The bacterial flagellum can be divided into three main parts: the transmembrane basal body that acts as a rotary motor as well as the flagellar protein export machine to construct the flagellar axial structures; the long filament extending into the cell exterior to function as a helical propeller; and the hook connecting the motor and filament as a universal joint to transmit motor torque to the filament. The Salmonella hook is a short, highly curved tubular structure built by helical assembly of about 120 copies of a single protein, FlgE. The length of the hook is regulated to 55 nm ± 7 nm, and its highly curved structure and bending flexibility make it work as a universal joint, transmitting motor torque to the filament regardless of the filament orientation off-axis of the motor during run and tumble of the cell for taxis. The FlgE molecule consists of three major domains, D0, D1 and D2, that are arranged radially from the inner core to the outer surface of the tubular structure and axially from the proximal to the distal end of the hook.

We carried out the structural analysis of the flagellar hook isolated from Salmonella in the straight form by cryoEM helical image analysis and built an atomic model based on the 4.1 Å resolution map. The hook was purified from a fliK-deficient mutant strain of Salmonella, SJW880, which produces polyhooks that are structurally identical to the native hook but can grow as long as 1 µm. The final resolution of the three-dimensional image reconstruction was 4.1 Å by the criteria of a Fourier shell correlation of 0.143. In the previous model built based on a cryoEM density map, the model of domain D0 was not so accurate and that of domain Dc was missing due to limited resolution of the density map. The model of Salmonella FlgE is now complete with the full-length chain connected from the N- to the C-terminus as shown in Figure 2 in two different views. Domain D0 consists of the N- and C-terminal α-helices (Ser 1–Ala 27 and Leu 367–Arg 402, respectively) forming an antiparallel coiled coil, with the C-terminal helix facing the central channel and tilted from the hook axis by about 17°. Domain Dc is a long β-hairpin (Lys 32–Phe 60) running parallel with the N-terminal helix and with its length nearly the same as that of the N-terminal helix. Thus, domains D0 and Dc together form a compact domain, which we hereafter call domain D0-Dc. In contrast, the Dc domains (green) have close interactions in the −5-start and 11-start helical lines, making a stable tubular structure, albeit the 6-start interactions are absent. Thus, the tubular structure of the hook is stabilized and maintained mainly by the intersubunit interactions of D0-Dc domains alone in the inner core of the hook structure. Residues 38–40 in the middle of the β-hairpin of domain Dc of subunit 0 are closely interacting with the tip loop (residues 328–331) of a short β-hairpin of domain D1 of subunit −5.

> SFSQAVSGLNAAATNLDVIGNNIANSATYGFKSGTASFADMFAGSKVGLGVKVAGITQDFTDGTTTNTGRGLDVAISQNGFFRLVDSNGSVFYSRNGQFKLDENRNLVNMQGMQLTGYPATGTPPTIQQGANPAPITIPNTLMAAKSTTTASMQINLNSTDPVPSKTPFSVSDADSYNKKGTVTVYDSQGNAHDMNVYFVKTKDNEWAVYTHDSSDPAATAPTTASTTLKFNENGILESGGTVNITTGTINGATAATFSLSFLNSMQQNTGANNIVATNQNGYKPGDLVSYQINNDGTVVGNYSNEQEQVLGQIVLANFANNEGLASQGDNVWAATQASGVALLGTAGSGNFGKLTNGALEASNVDLSKELVNMIVAQRNYQSNAQTIKTQDQILNTLVNLR> EL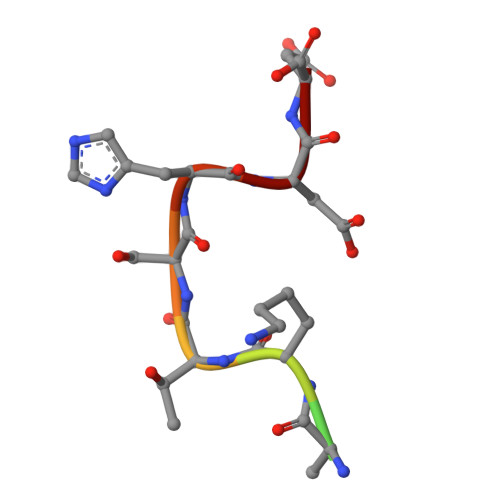VIKTSHDD>MAGDTTITIVGNLTADPELRFTSSGAAVVNFTVASTPRIYDRQSGEWKDGEALFLRCNIWREAAENVAESLTRGARVIVTGRLKQRSFETREGEKRTVVEVEVDEIGPSLRYATAKVNKASRSGGGGGGFG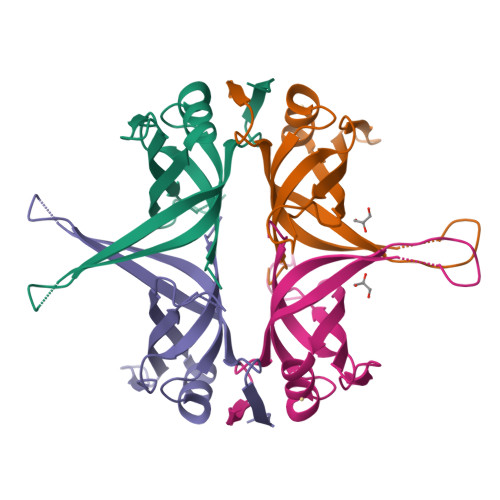SGSRQAPAQMSGGVGDDPWGSAPTSGSFGVGDEEPPF[2x]> SNAMTDIRKAATLVVIRDGANKDIEVLVVRRAKTMRFLPGFVAFPGGAADPSDAEMA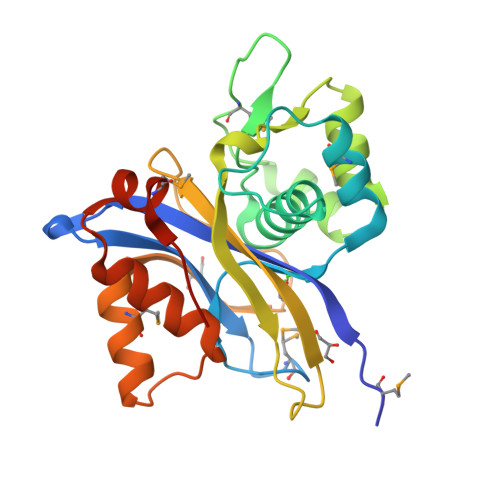KRAFGRPVCAEDDDDPALAVTALRETAEEIGWLLAVRDGEGTKMDTPLAPDEQADLCKGGDALSAWLSARGLAFDLGLLRRIGRFVTPPTQPVRFDTRFFLCVGQHLGEPRLHGAELDAALWTPARDMLTRIQSGELPAVRPTIAVLKALVACPNAEIAMSTLSIGPLPPPAPRA>CCG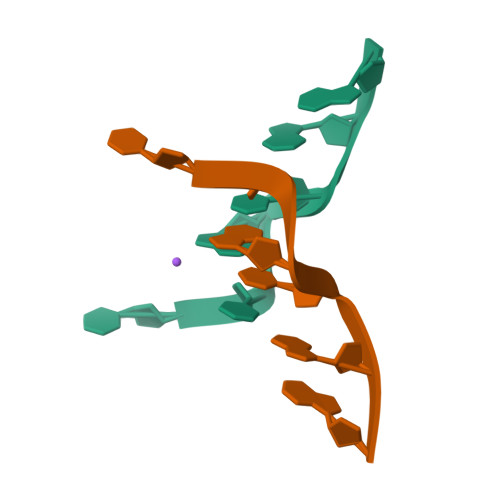CGG[2x]> MATLSLTVNSGDPPLGALLAVEHVKDDVSISVEEGKENILHVSENVIFTDVNSILRYLARVATTAGLYGSNLMEHTEIDHWLEFSATKLSSCDSFTSTINELNHCLSLRTYLVGNSLSLADLCVWATLKGNAAWQEQLKQKKAPVHVKRWFGFLEAQQAFQSVGTKWDVSTTKA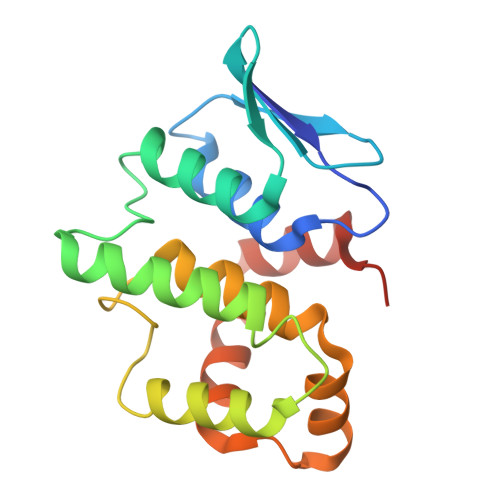R> GHLTSSNALRGDAHSRLAAHRGLLERTSRTTRVAGILRDAIIDGTFRPGARLSEPDICAALDVSRNTVREAFQILIEDRLVAHELNRGVFVRVPTAEDITELYICRRVVECAGVNGFDPATGDLSRVA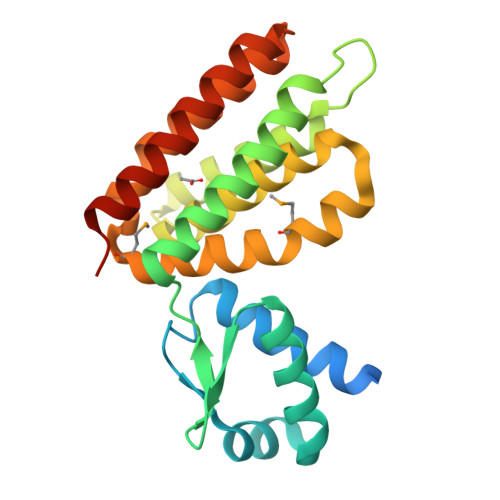EALDLADERYAVEDWTGVGTADIHFHSALASLNNSNRIDELMRSVWNEARLVFHVMDDAHRFHGPYLTRNHEIYDALAAGNTEAAGQLLKTYLEDAEAQILGAYRPVSGGS(3S)-3-cyclopentyl-3-[4-(7H-pyrrolo[2,3-d]pyrimidin-4-yl)-1H-pyrazol-1-yl]propanenitrile 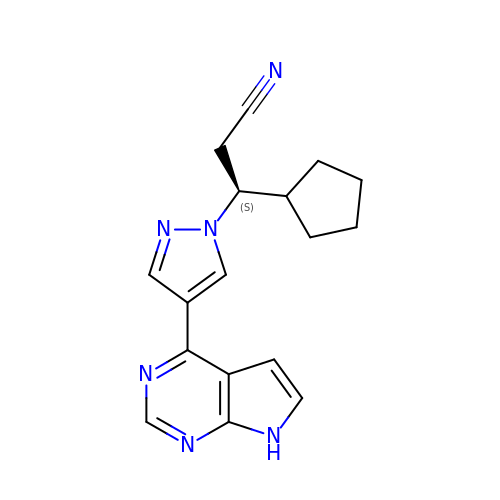| C17 H18 N6 | HFNKQEVNSGCOJV-HNNXBMFYSA-N> MKTEFSGDTDAVHGKTHVFIRSIKNGSHMQEAKIDIKSLYDSLAKKYDVQHK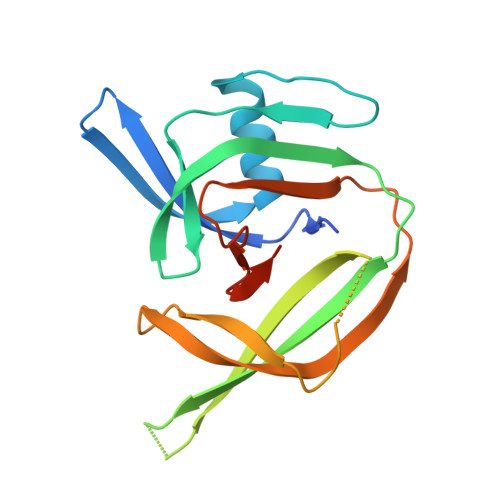NSYEVIYPKGYEIKVLGNKYVKLVAMSRHKTQKHLVKIVVKSEKTIDSLDPIRQKSLLKKQDEVVVTTDHIAMVYNDDHFFENVNAKNLKVGNYVSVYDEASDKEVIGEIASIEDLGMTDDYVYDAEVDDDSHAFYASNILVHASQFCNGTKLGG> GEDEIESAGVSASEVESSATKQKVALHPHD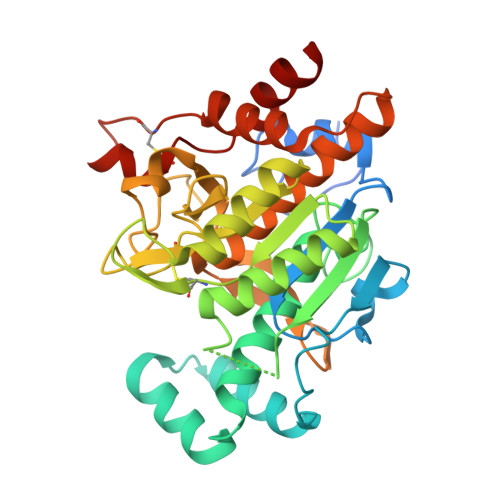LDERIPGLADLHNQTLGDPQITIVIIDGDPDYTLSCFEGAEVSKVFPYWHEPAEPITPEDYAAFQSIRDQGLKGKEKEEALEAVIPDTKDRIVLNDAACHVTSTIVGQEHSPVFGIAPNCRVINMPQDAVIRGNYDDVMSPLNLARAIDLALELGANIIHCAFCRPTQTSEGEEILVQAIKKCQDNNVLIVSPTGNNSNESWCLPAVLPGTLAVGAAKVDGTPCHFSNWGGNNTKEGILAPGEEILGAQPCTEEPVRLTGTSMAAPVMTGISALLMSLQVQQGKPVDAEAVRTALLKTAIPCDPEVVEEPERCLRGFVNIPGAMKVLFGQ>MMIRG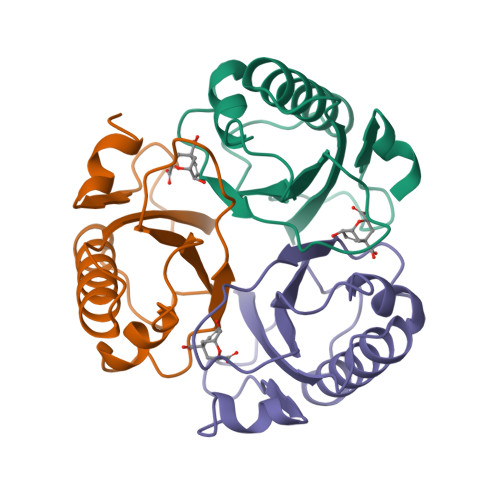IRGATTVERDTEEEILQKTKQLLEKIIEENHTKPEDVVQMLLSATPDLHAVFPAKAVRELSGWQYVPVTCMQEMDVTGGLKKCIRVMMTVQTDVPQDQIRHVYLEKAVVLRPDLSLTKNTEL[12x]> DPTMVSVIKPEMKMRY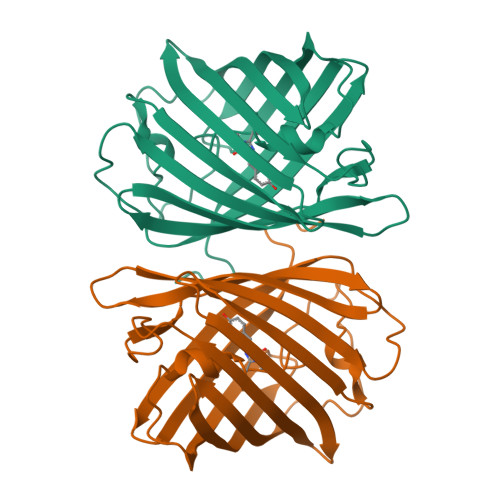YMDGSVNGHEFTVEGEGTGRPYEGKQKITLDVTKGGPLPFAFDLLSTVFSYGNRALTKYPDDIPDYFKQCFPGGYSWERKFEFEDGGLAIAKAEISLKGNCFEHKSTIEGTFPDSSPIMQNKTLGWEPSTEKMTVRDGSMKGDDASYLKLVGGGNHKCYFTTTYTAKKKIPNLPGSHFIGHRISSVVEGTKIKVMEDAIAHLYPFNGS>[2x]SMDHYKAKATRHIFLIRHSQYHVDGSL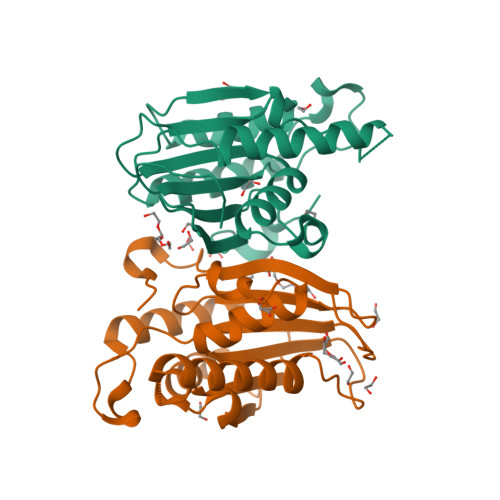EKDRTLTPLGREQAELTGLRLASLGLKFNKIVHSSMTRAIETTDIISRHLPGVCKVSTDLLREGAPIEPDPPVSHWKPEAVQYYEDGARIEAAFRNYIHRADARQEEDSYEIFICHANVIRYIVCRALQFPPEGWLRLSLNNGSITHLVIRPNGRVALRTLGDTGFMPPDKITRS>[2x]GPGGTMGRVTAPEPLSAFHQVAEFVSGEAVLDDWLKQKGLKNQALGAARTFVVCKKDTKQVAGFYSLATGSVNHTEATGNLRRNMPDPIPVIILARLAVDLSFHGKGLGADLLHDAVLRCYRVAENIGVRAIMVHALTEEAKNFFIHHGFKSSQTQQRTLFLRLPQ

Here we reveal that one such toxin, TacT, is an acetyltransferase that blocks the primary amine group of amino acids on charged tRNA molecules, thereby inhibiting translation and promoting persister formation. Class II TA operons encode a non-secreted toxin, which inhibits an essential cellular function such as RNA translation or DNA replication, and an antitoxin, which interacts with and neutralizes the toxin. GNAT superfamily enzymes catalyze acetyl group transfer from acetyl-coenzyme A (Ac-CoA) to a wide range of substrates. Here we show that bacteria can acetylate the amino acid on charged tRNA molecules through the activity of TacT, an atypical acetyltransferase that displays unique structural features including two positively charged patches at its surface that are essential for toxicity.

We designed single amino acid substitutions of predicted Ac-CoA binding residues intending to block Ac-CoA binding (A93P) or to allow binding to Ac-CoA but prevent transfer of the acetyl moiety to the acceptor molecule (Y140F). The conserved Y140 natively coordinates an oxygen atom of Ac-CoA to ensure correct orientation of the acetyl group for transfer. We then purified the non-toxic T8Y140F mutant protein, which can be produced in large quantities in the absence of its antitoxin A8, and solved its crystal structure to 1.7 Å resolution. The asymmetric unit of the crystals contains a dimer of T8 with an extensive dimeric interface burying a total of 4,739 Å2 of surface area. The T8 monomer consists of an acetyltransferase fold, and an Ac-CoA molecule is clearly visible in the electron density of the active site. Compared to that of other acetyltransferases, the structure contains two unique features: an extension to the α3 helix and longer, curved β2 and β3 strands with an insertion of short 310- and α helices (η1 and α2) between them. The dimer interface is also unique and critically depends on both the α3 and β2-β3 extensions. Hydrophobic sidechains from these structural components and from the α1-β1 loop are buried to stabilize the dimer in conjunction with several hydrogen bonds. Examination of the surface electrostatic potential of the TacT dimer revealed a positively charged groove leading from the active site of one monomer to an extra patch of positive charge around the α2 region of the second molecule of the dimer. We modeled the coupled acceptor stem of the phosphodiester backbone lying in the groove with phosphate groups interacting with the sidechains of Arg-91, Lys-33, and Lys-36 and the positive surface of the α2 region positioned to interact with phosphates from the remainder of the tRNA molecule, with sidechains of Arg-77, Arg-78, Lys-146, and Arg-158 involved.>MKSRTACKRCRLK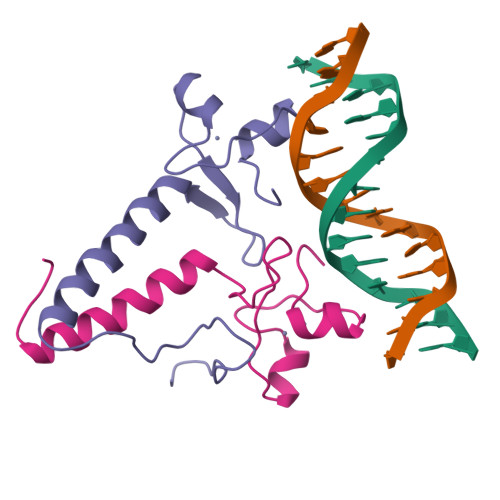KIKCDQEFPSCKRCAKLEVPCVSLDPATGKDVPRSYVFFLEDRLAVMMRVLKEYGVDPTKIRGNIPATSDDEPFDLKKYSSVS[2x]>[3x]KTVQVTLHAVETDVAYDNKGSTYRAWTFDGKVPGPVVRV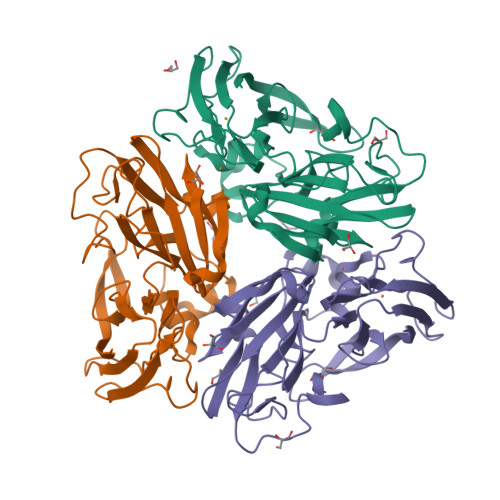TEGDTVEFTLINDKNSKNSHSMDFHAARLDVVEDFESIKPGETKKYTFTADNPGVFFYHCGSDPMIQHIARGMYGVIIVDPKDANALPKADREYVLIQAEHYENPDDKTAMMQNKWSNVVFNGGVFKYDPVHDSEATSWLQAKPGERVRIYFVNAGPNELSSLHPIAGIWDRVYPSGNPKNVQYALQSYLIGAGDAATLDLISPVEGANAIVDHSMRHAHSGAIAVIMFTNDADPEAGRGENILIR> EIPLKYGATNEGKRQDPAMQKFRDNRLGAFIHWGLYAIPGGEWNGKVYGGAAEWLKSWAKVPADEWLKLMDQWNPTKFDAKKWAKMAKEMGTKYVKITTKHHEGFCLWPSKYTKYTVANTPYKRDILGELVKAYNDEGIDVHFYFSVMDWSNPDYRYDIKSKEDSIAFSRFLEFTDNQLKELATRYPTVKDFWFDGTWDASVKKNGWWTAHAEQMLKELVPGVAINSRLRADDKGKRHFDSNGRLMGDYESGYERRLPDPVKDLKVTQWDWEACMTIPENQWGYHKDWSLSYVKTPIEVIDRIVHAVSMGGNMVVNFGPQADGDFRPEEKAMATAIGKWMNRYGKAVYACDYAGFEKQDWGYYTRGKNDEVYMVVFNQPYSERLIVKTPKGITVEKATLLTTGEDITVVETTRNEYNVSVPKKNPGEPYVI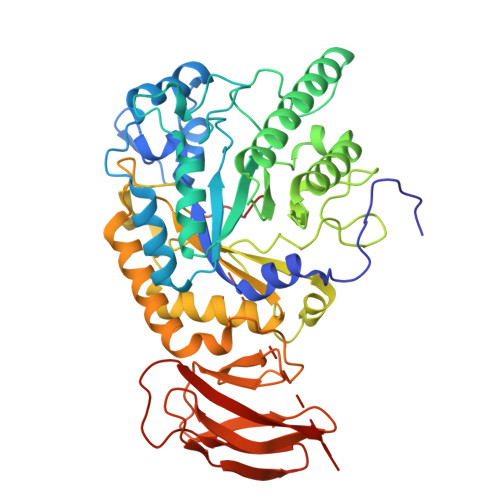QLKVRAAKGTKSLYRDALT> PELPEVETVRRELEKRIVGQKIISIEATYPRMVLTGFEQLKKELTGKTIQGISRRGKYLIFEI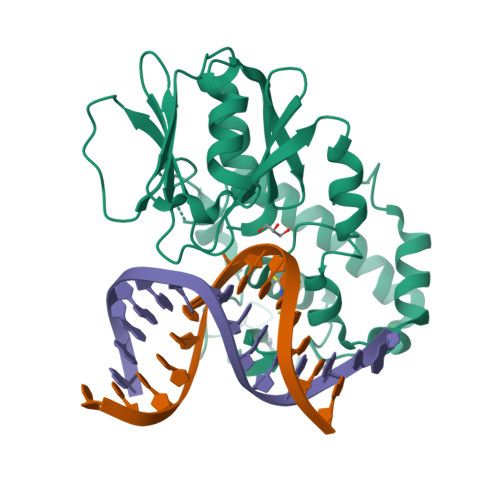GDDFRLISHLRMEGKYRLATLDAPREKHDHLTMKFADGQLIYADVRKFGTWELISTDQVLPYFLKKKIGPEPTYDEDFDEKLFREKLRKSTKKIKPYLLEQTLVAGLGNIYVDEVLWLAKIHPEKETNQLIESSIHLLHDSIIEILQKAIKLGGSSIRTYSALGSTGKMQNELQVYGKTGEKCSRCGAEIQKIKVAGRGTHFCPVCQQK> LGRTTRDDLINGNSASCADVIFIYARGSTETGNLGTLGPSIASNLESAFGKDGVWIQGVGGAYRATLGDNALPRGTSSAAIREMLGLFQQANTKC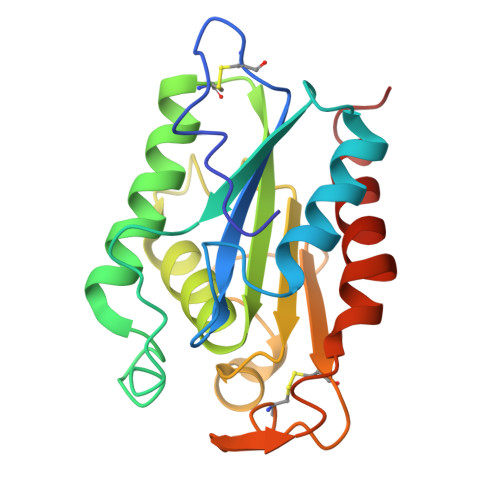PDATLIAGGYSQGAALAAASIEDLDSAIRDKIAGTVLFGYTKNLQNRGRIPNYPADRTKVFCNTGDLVCTGSLIVAAPHLAYGPDARGPAPEFLIEKVRAVRGSA> QTQQEEEEEDEDHGPDDYDEEDEDEVEEEETNRLPGGRSRVLLRCYTCKSLPRDERCDLTQDCSHGQTCTTLIAHGNTESGLLTTHSTWCTDSCQPITKTVEGTQVTMTCCQS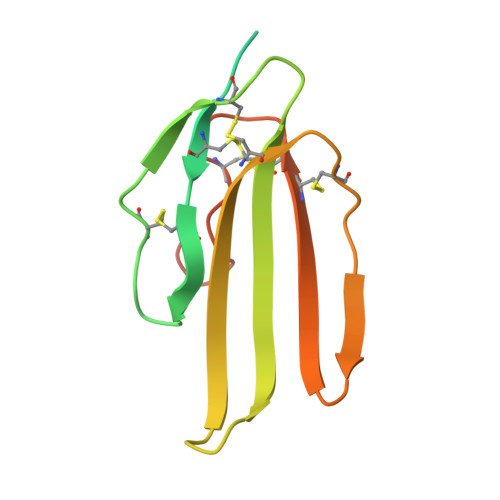SLCNVPPWQSSRVQDPTG> MGSSHHHHHHSSGRENLYFQGSTALRPYHDVLSQWQRHYNADRNRWHSAWRQANSNNPQIETRTGRALKATADLLEDATQPGRVALELRSVPLPQFPDQAFRLSHLQHMTIDAAGLMELPDTMQQFAGLETLTLARNPLRALPASIASLNRLRELSIRACPELTELPEPLASTDASG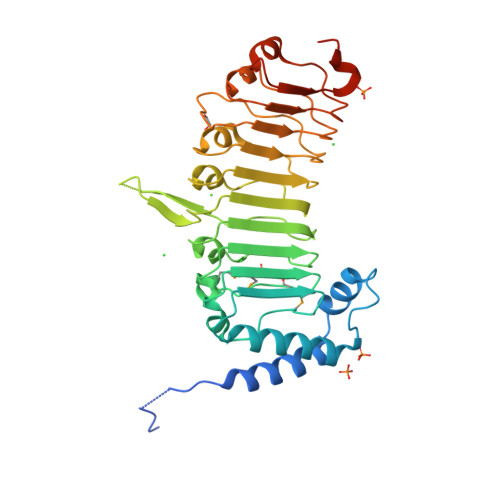EHQGLVNLQSLRLEWTGIRSLPASIANLQNLKSLKIRNSPLSALGPAIHHLPKLEELDLRGCTALRNYPPIFGGRAPLKRLILKDCSNLLTLPLDIHRLTQLEKLDLRGCVNLSRLPSLIAQLPANCIILVPPHLQAQLDQHRPVARPAEP> MSGTANSRRKEVLRVPVIDLNRVSDEEQLLPVVRAILLQHDTFLLKNYANKAVLDALLAGLTTKDLPDTSQGFDANFTGTLPLEDDVWLEQYIFDTDPQLRFDRKCRNESLCSIYSRLFKLGLFFAQLCVKSVVSSAELQDCISTSHYATKLTRYFNDNGSTHDGADAGATVLPTGDDFQYLFERDYVTFLPTGVLTIFPCAKAIRYKPSTMATTDNSWVSIDEPDCLLFHTGTLLARWSQGMHTTSPLQIDPRANIVSLTIWPPLTTPISSKGEGTIANHLLEQQIKAFPKVAQQYYPRELSILRLQDAMKFVKELFTVCETVLSLN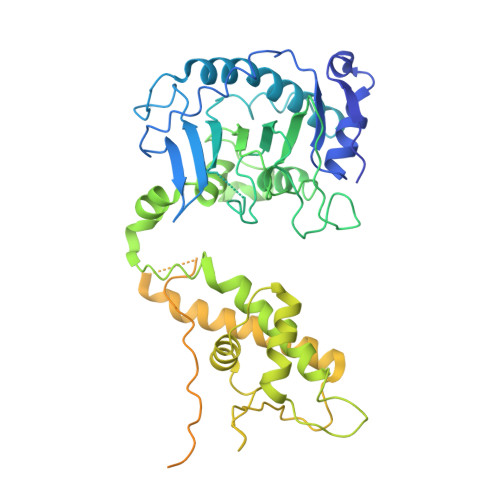ALSRSTGVPPELHVLLPQISSMMKRKIVQDDILKLLTIWSDAYVVELNSRGELTMNLPKRDNLTTLTNKSRTLAFVERAESWYQQVIASKDEIMTDVPAFKINKRRSSSNSKTVLSSKVQTKSSNANALNNSRYLANSKENFMYKEKMPDSQANLMDRLRERERRSAALLSQRQKRYQQFLAMKMTQVFDILFSLTRGQPYTETYLSSLIVDSLQDSNNPIGTKEASEILAGLQGILPMDISVHQVDGGLKVYRWNSLDKNRFSKLLQIHKSKQQD Echistatin (Ech) is a short disintegrin isolated from Echis carinatus that contains 49 residues with 4 disulfide bonds. Ech is the most extensively characterized disintegrin and has a conserved RGD motif and a long C-terminal NPHKGPAT tail. Similar to the reported structures of other disintegrins, Ech has a well-defined core composed of a series of nonclassical turns crosslinked by disulfide bonds (C2-C11, C7-C32, C8-C37, and C20-C39). The RGD motif is located in a protruding loop that is formed by two antiparallel β-strands (residues 16–20 and 29–31).

The diffraction data of Ech were obtained to a resolution of 1.80 Å from a single frozen crystal, which contained two molecules per asymmetric unit. Superimposition of the backbones of chains A and B with an RMSD value of 0.226 Å demonstrated that their overall structures were very similar, except for the RGD loop and C-terminal loop. Structural analysis showed that the RGD loop of chain B was squeezed by residues K21, R41, and K45 in contact with sulfate ions and residue S4 of chain A through crystal packing. Therefore, the R and D side chains of the chain B structure interacted with each other and formed hydrogen bonds. In contrast to chain B, the R and D side chains in the RGD loop of chain A are far from each other. Furthermore, the backbones of the C-terminal GPAT residues of chain A showed a weaker electron density map. In contrast, the conformation of the C-terminal tail of Ech chain B was well defined, possibly because the C-terminal residue K45 can interact with the O atoms of SO42-. The structural analysis of Ech chains A and B showed that the side chain of the D30 residue in the RGD loop and the amide proton of the N42 residue in the C-terminus formed hydrogen bonds. Interestingly, the carboxyl group of residue M28 interacts with the side-chain Nζ proton of residue K45, and the side chain of residue D30 interacts with the side chain Nζ proton of residue K45, resulting in a unique turn structure for Ech. These results showed that the K45 residue stabilizes the conformation of Ech’s C-terminus and is important for its integrin recognition.

>EFECESGPCCRNCKFLKEGTICKRARGDDMDDYCNGKTCDCPRNPHKGPAT[2x]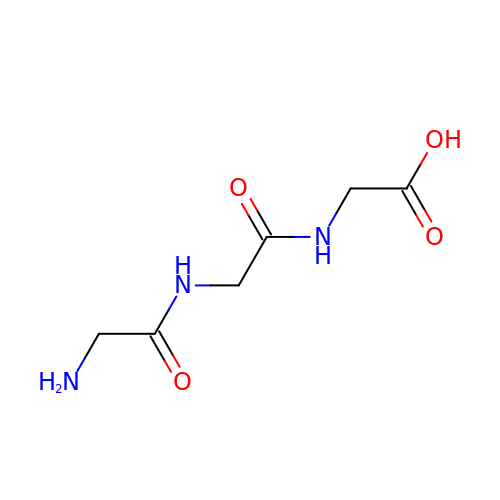glycylglycylglycine | C6 H11 N3 O4 | XKUKSGPZAADMRA-UHFFFAOYSA-N> MTVAYSLENLKKISNSLVGDQLAKVDYFLAPKCQIFQCLLSIEQSDGVELKNAKLDLLYTLLHLEPQQRDIVGTYYFDIVSAIYKSMSLASSFTKNNSSTNYKYIKLLNLCAGVYPNCGFPDLQYLQNGFIQLVNHKFLRSKCKIDEVVTIIELLKLFLLVDEKNCSDFNKSKFMEEEREVTETSHYQDFKMAESLEHIIVKISSKYLDQISLKYIVRLKVSRPASPSSVKNDPFDNKGVDCTRAIPKKINISNMYDSSLLSLALLLYLRYHY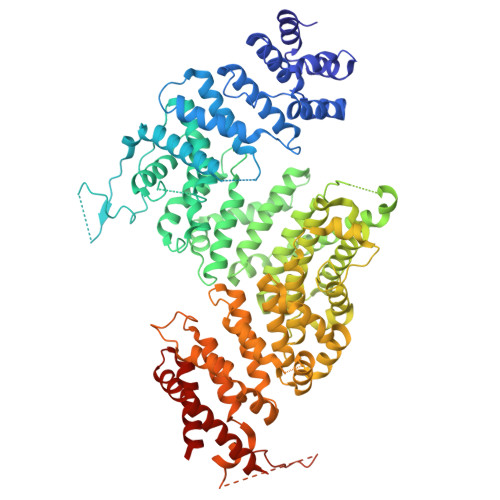MIPGDRKLRNDATFKMFVLGLLKSNDVNIRCVALKFLLQPYFTEDKKWEDTRTLEKILPYLVKSFNYDPLPWWFDPFDMLDSLIVLYNEITPMNNPVLTTLAHTNVIFCILSRFAQCLSLPQHNEATLKTTTKFIKICASFAASDEKYRLLLLNDTLLLNHLEYGLESHITLIQDFISLKDEIKETTTESHSMCLPPIYDHDFVAAWLLLLKSFSRSVSALRTTLKRNKIAQLLLQILSKTYTLTKECYFAGQDFMKPEIMIMGITLGSICNFVVEFSNLQSFMLRNGIIDIIEKMLTDPLFNSKKAWDDNEDERRIALQGIPVHEVKANSLWVLRHLMYNCQNEEKFQLLAKIPMNLILDFINDPCWAVQAQCFQLLRNLTCNSRKIVNILLEKFKDVEYKIDPQTGNKISIGSTYLFEFLAKKMRLLNPLDTQQKKAMEGILYIIVNLAAVNENKKQLVIEQDEILNIMSEILVETTTDSSSYGNDSNLKLACLWVLNNLLWNSSVSHYTQYAIENGLEPGHSPSDSENPQSTVTIGYNESVAGGYSRGKYYDEPDGDDSSSNANDDEDDDNDEGDDEGDEFVRTPAAKGSTSNVQVTRATVERCRKLVEVGLYDLVRKNITDESLSVREKARTLLYHMDLLLKVK>LKESPSGYLRSGEGDTGCGELVWVGEPLTLRTAETITGKYGVWMRDPKPTYPYTQETTWRIDTVGTDVRQVFEYDLISQFMQGYPSKVHILPRPLESTGAVVYSGSLYFQGA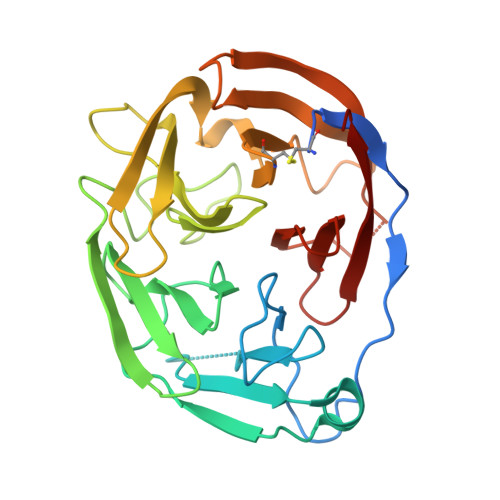ESRTVIRYELNTETVKAEKEIPGAGYHGQFPYSWGGYTDIDLAVDEAGLWVIYSTDEAKGAIVLSKLNPENLELEQTWETNIRKQSVAEAFIICGTLYTVSSYTSADATVNFAYDTGTGISKTLTIPFKNRYKYSSMISYNPLEKKLFAWDNLNMVTYDIKLSKM[2x]The cyanobacterium Prochloron spp. produces multiple macrocyclic cyanobactins, which are known as the trunkamides (seven or eight residues) and the patellamides (eight residues). These natural products originate from two different ribosomal precursor peptides (denoted TruE and PatE), and each ribosomal peptide contains multiple distinct core peptides. Heterocyclization of the multiple cysteine residues in TruE is carried out by the single enzyme, TruD, which by definition is processive. We show by biochemical assay that TruD is an adenylase, not a kinase, and that TruD processes cysteines in a defined order, which we describe. We have shown that the leader sequence (crucially residues 26–37) is required for processivity (heterocyclization of subsequent cysteines).

Domains 1 and 2 of TruD share 21 % sequence identity and structural fold with the enzyme MccB, an adenylase found in the microcin C7 antibiotic production pathway (MccB catalyzes two successive adenylation reactions). Pairwise superposition of TruD with the MccB structure gives a Cα rmsd of 5.4 Å over 219 structurally equivalent residues (MccB lacks the third domain); individual domain superpositions are much lower due to a domain rotation (2.6 Å over 80 residues and 2.0 Å over 152 residues). TruD and MccB possess a similar dimeric arrangement and both share two CXXC motifs in domain 2 that bind a Zn2+ ligated in a tetrahedral arrangement of sulfur atoms. Both motifs are conserved in cyanobactin heterocyclases and these motifs (and associated zinc) are a conserved feature of one class of adenylating enzymes. The coordinatively saturated zinc plays a structural role only12b, in this class of adenylating enzymes. Domain 2 of TruD shares the fold of this class of adenylating enzymes; other members include human ubiquitin-activating enzyme 5 (1.9 Å rmsd over 134 Cαs) and thiamine pyrophosphate biosynthetic enzyme ThiF (2.1 Å over 142 Cαs). There is, however, a subtle topology difference; all the adenylating enzymes that share a fold with TruD have an insertion between the first and second strand of the central β-sheet relative to TruD domain 2. Significantly this means that the ATP binding site of MccB is not fully conserved in TruD. Domain 3 of TruD is a novel fold and has a large negatively charged central cleft. Structural data of course do not establish the mechanism but they are entirely consistent with TruD being an adenylase enzyme.

> GQPTALQIKPHFHVEIIEPKQVYLLGEQGNHALTGQLYCQILPFLNGEYTREQIVEKLDGQVPEEYIDFVLSRLVEKGYLTEVAPELSLEVAAFWSELGIAPSVVAEGLKQPVTVTTAGKGIREGIVANLAAALEEAGIQVSDPRDPKAPKAGDSTAQLQVVLTDDYLQPELAAINKEALERQQPWLLVKPVGSILWLGPLFVPGETGCWHCLAQRLQGNREVEASVLQQKRALQERNGQNKNGAVSCLPTARATLPSTLQTGLQWAATEIAKWMVKRHLNAIAPGTARFPTLAGKIFTFNQTTLELKAHPLSRRPQCPTCGDRETLQRRGFEPLKLESRPKHFTSDGGHRAMTPEQTVQKYQHLIGPITGVVTELVRISDPANPLVHTYRAGHSFGSATSLRGLRNVLRHKSSGKGKTDSQSRASGLCEAIERYSGIFQGDEPRKRATLAELGDLAIHPEQCLHFSDRQYDNRESSNERATVTHDWIPQRFDASKAHDWTPVWSLTEQTHKYLPTALCYYRYPFPPEHRFCRSDSNGNAAGNTLEEAILQGFMELVERDSVCLWWYNRVSRPAVDLSSFDEPYFLQLQQFYQTQNRDLWVLDLTADLGIPAFVGVSNRKAGSSERIILGFGAHLDPTVAILRALTEVNQIGLELDKVSDESLKNDATDWLVNATLAASPYLVADASQPLKTAKDYPRRWSDDIYTDVMTCVEIAKQAGLETLVLDQTRPDIGLNVVKVIVPGMRFWSRFGSGRLYDVPVKLGWREQPLAEAQMNPTPMPF>[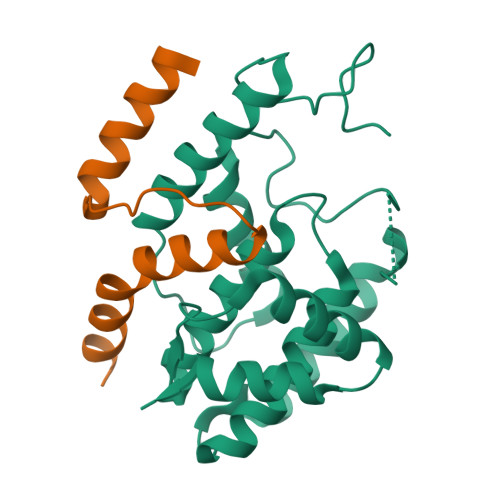3x]MGSSHHHHHHSQDPNSSSARLQVEMGDKFGEGRDPYLYPGLDIMRNRLNIHQQQRLEQAAYEMTALRAATIELGPLVRGLPHLRTIHRQLYQDIFDWAGQLREVDIYQGDTPFCHFAYIEKEGNALMQDLEEEGYLVGLEKAKFVERLAHYYCEINVLHPFRVGSGLAQRIFFEQLAIHAGYQLSWQGIEKEAWNQANQSGAMGDLTALQMIFSKVVSEAGESE;>MAYPYDVPDYAAAVKKLTDKQKSRLWELQRNRNFQASRRLGGVEMPLVTLTAAEALARLEELRSHYER[3x]>[3x]MHHHHHHENLYFQGSTSENITQKVVWVEESDKRSFLLDLLNATGKDSLTLVFVETKKGADSLEDFLYHEGYACTS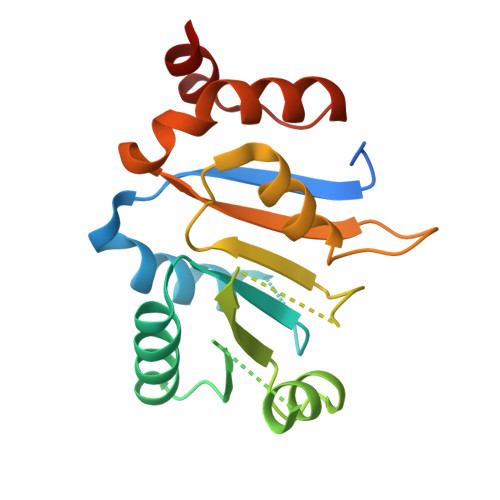IHGDRSQRDREEALHQFRSGKSPILVATAVAARGLDISNVKHVINFDLPSDIEEYVHRIGRTGRVGNLGLATSFFNERNINITKDLLDLLVEAKQEVPSWLENMAYEHHY> VERLQIFQHLH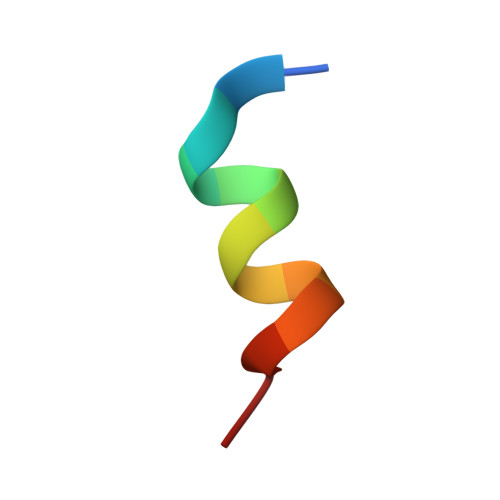PI> ASMTGGQQMGRDQAGITGTWYNQLGSTFIVTAGADGALTGTYVTARGNAESRYVLTGRYDSAPATAGSGTALGWTVAWKNNYRNAHSATTWSGQYVGGAEARINTQWLLTSGTTEANAWRSTLVGHD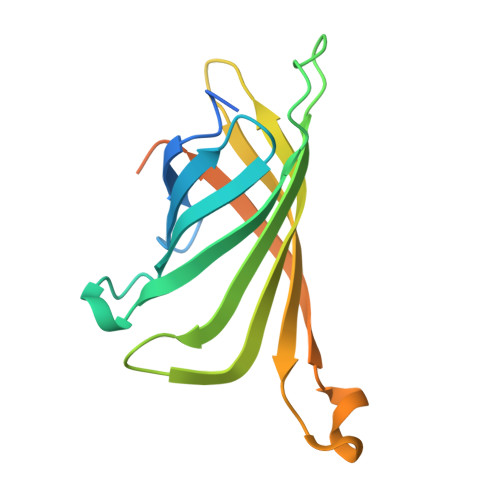TFTKVQPSAASIDAAKKAGVNNGNPLDAVQQ>[4x]GPHMTELLFNKRLQVLVKSKDTDERRSVIRVSIELQLPSSPVHRKDLVVRLTDDTDLYFLYNLIISEEDFQSLKVQQGLLIDFTSFPQKFIDLLEQCICE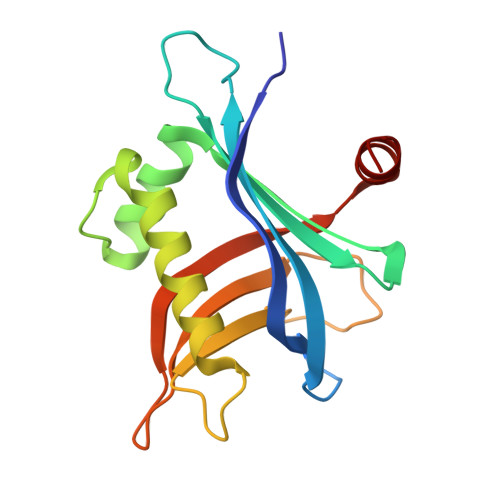QDKENPRFLLQLSSSSSAFDHSPSNLNIVETNAFKHLTHLSLKLLPGSDTDIKKYLASC> GPDSMADITDKTAEQLENLNIQDDQKQAATGSESQSVENSSASLYVGDLEPSVSEAHLYDIFSPIGSVSSIRVCRDAITKTSLGYAYVNFNDHEAGRKAIEQLNYTPIKGRLCRIMWSQRDPSLRKKGSGNIFIKNLHPDIDNKALYDTFSVFGDILSSKIATDENGKSKGFGFVHFEEEGAAKEAIDALNGMLLNGQEIYVAPHLSRKERDSQLEETKAHYTNLYVKNINSETTDEQFQELFAKFGPIVSASLEKDADGKLKGFGFVNYEKHEDAVKAVEALNDSELNGEKLYVGRAQKKNERMHVLKKQYEAYRLEKMAKYQGVNLFVKNLDDSVDDEKLEEEFAPYGTITSAKVMRTENGKSKGFGFVCFSTPEEATKAITEKNQQIVAGKPLYVAIAQRKDVRRSQLAQQIQARNQMRYQQATAAAAAAA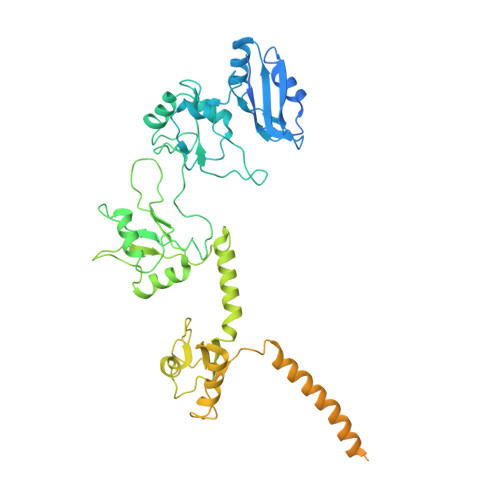AGMPGQFMPPMFYGVMPPRGVPFNGPNPQQMNPMGGMPKNGMPPQFRNGPVYGVPPQGGFPRNANDNNQFYQQKQRQALGEQLYKKVSAKTSNEEAAGKITGMILDLPPQEVFPLLESDELFEQHYKEASAAYESFKKEQEQQTEQA> MSTARPRIITSKAPLLPQQTTPEQRYWRQYTS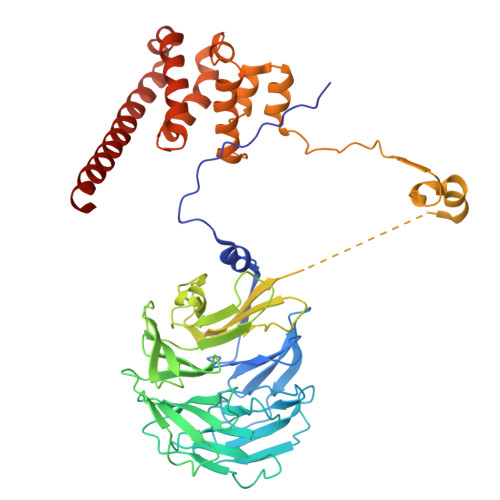AQLVKEHNSVTHISFNPQHPHDFAVTSSTRVQIFSSRTRQVIKTFSRFKDVVYSASFRSDGKLLCAGDATGLVSVYDSYNPRTILLSINASTHPTHVTKFHTQDNKILATASDDRVTRLWDISNAYEPQLELTGATDYVRTLSFIPAAPHLVATGSYDGLIRLYDTRSSGSTPIYSLNHDQPVENVIAVSPTQIVSCGGNNFKVWDLTSNKKLYERGNFNKAVTCLDYVENFDSPMQSALIASSLDGHVKVFDPLDNFQVKFGWKFSGPVLSCAVSPSTAQGNRHLVAGLSSGLLAIRTKKKEKRSSDKENAPASFNKNAKSNNFQRMMRGSEYQGDQEHIIHNDKVRSQRRMRAFERNINQFKWSEALDNAFVPGMAKELTLTVLQELRKRGKVRVALYGRDESTLEPLLNWCLKGIEDVRSASIVADWVAVVLELYGNTLESSPVLQELMIDLKTKVRHEIHKSKEAQRIEGMLQLLTS> MKHHHHHHHMVSTLKPLKIGKHTIKFPIFQGGMGVGISWDELAGNVAKEGALGVISAVGTGYYKNMRFVERIVAKKPFEALNFYSKKALNEIFANARKICGNNPLGANILYAINDYGRVLRDSCEAGANIIITGAGLPTNMPEFAKDFSDVALIPIISSAKALKILCKRWSDRYKRIPDAFIVEGPLSGGHQGFKYEDCFKEEFRLENLVPKVVEASKEWGNIPIIAAGGIWDRKDIDTMLSLGASGVQMATRFLGTKECDAKVYADLLPTLKKEDILLIKSPVGYPARAINTGVIKRIEEGNAPKIACVSNCVAPCNRGEEAKKVGYCIADGLGRSYLGNREEGLYFTGANGYRVDKIISVHELIKELTEG

The bifunctional dehydrogenase/isomerase FabX is an essential UFA biosynthesis enzyme in the widespread human pathogen Helicobacter pylori, a bacterium etiologically related to 95% of gastric cancers. FabX belongs to the nitronate monooxygenase (NMO) flavoprotein family but contains an atypical [4Fe-4S] cluster absent in all other family members characterized to date. We demonstrate that the [4Fe–4S] cluster functions as a temporary electron depot that receives electrons from FMN and sends electrons back to FMN to achieve independent bidirectional internal electron transfer.

We solved the crystal structure of FabX at 1.7 Å resolution with a single FabX monomer observed in the asymmetric unit. The overall structure of FabX predominantly consists of a large canonical TIM-barrel fold subdomain at its N-terminus (residues from 1 to 266, including β1–β8 and α1–α11). It contains a FMN cofactor-binding core that consists of eight continuous β-strand–α-helix repeats (β3–α5–β4–α6–β5–α7–β6–α8), and a FMN molecule is noncovalently bound inside the core. In contrast, the catalytic residue H182 is located ~6.5 Å from the FMN cofactor, and is stabilized through hydrogen bonding with the sidechain of S273. Moreover, the H182 nitrogen atoms of the sidechain (Nδ1) and backbone (N) together with four nitrogen atoms (N1, N3, N5, and N10) of FMN form a positive charged oxyanion hole located between the H182 sidechain and the FMN cofactor, which has never been observed in this family. A chloride anion was found locked in the oxyanion hole and is stabilized through hydrogen bonds with E175 and G180 mediated by nearby water chains. In addition to the canonical TIM-barrel fold core, FabX was unexpectedly found to contain a small [4Fe–4S] cluster-binding subdomain at its C-terminus (residues from 267 to 363), which has never been observed in enzymes involved in the fatty acid synthesis. The subdomain consists of six α‐helices and two β‐strands (α12–α17 and β9–β10), and four cysteine residues C300, C304, C308 and C320 hold the [4Fe–4S] cluster, a second electron transfer component other than FMN, through coordination bonding interactions. The FMN core is located near the kink of the tunnel, whereas the [4Fe–4S] cluster is located at the end of the tunnel where it blocks the end, and is 13.4 Å away from the FMN cofactor (nearest atoms distance), which is within the theoretical distance limitation (<14 Å) that electrons can directly transfer.> MWF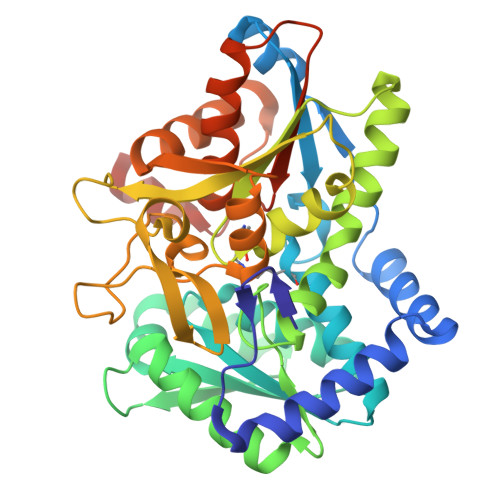GEFGGQYVPETLIEPLKELEKAYKRFKDDEEFNRQLNYYLKTWAGRPTPLYYAKRLTEKIGGAKIYLKREDLVHGGAHKTNNAIGQALLAKFMGKTRLIAETGAGQHGVATAMAGALLGMKVDIYMGAEDVERQKMNVFRMKLLGANVIPVNSGSRTLKDAINEALRDWVATFEYTHYLIGSVVGPHPYPTIVRDFQSVIGREAKAQILEAEGQLPDVIVACVGGGSNAMGIFYPFVNDKKVKLVGVEAGGKGLESGKHSASLNAGQVGVFHGMLSYFLQDEEGQIKPTHSIAPGLDYPGVGPEHAYLKKIQRAEYVTVTDEEALKAFHELSRTEGIIPALESAHAVAYAMKLAKEMSRDEIIIVNLSGRGDKDLDIVLKVSGNVLEHHHHHH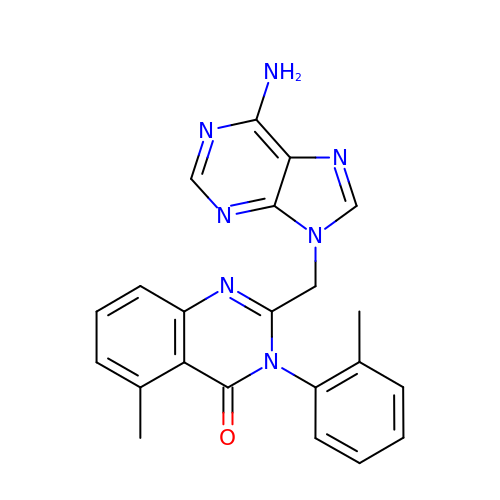2-[(6-AMINO-9H-PURIN-9-YL)METHYL]-5-METHYL-3-(2-METHYLPHENYL)QUINAZOLIN-4(3H)-ONE | C22 H19 N7 O | GNWHRHGTIBRNSM-UHFFFAOYSA-N>GPLGSDEKKKYTLLAKVTGLERFGSATGKKENPTIIFDCSTNLPTFRKQQYKNVKKSYEEFHQLFKYLNVAIQESFVPTLPSAYTTFGINSEEDRMKVTRNFQLWFNRL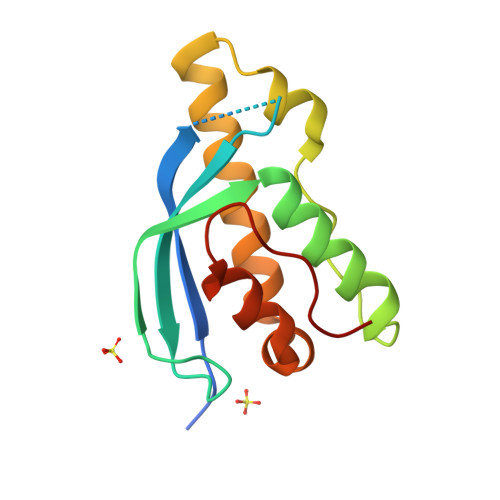SQDPLIIRNEEVAFFIESDFNTYTPINKSK[2x]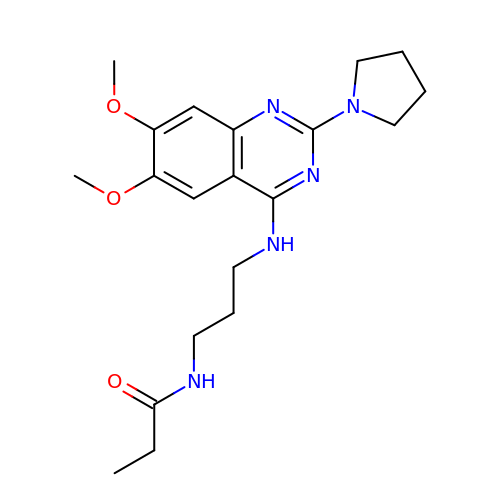N-(3-{[6,7-dimethoxy-2-(pyrrolidin-1-yl)quinazolin-4-yl]amino}propyl)propanamide | C20 H29 N5 O3 | GDDIMJLTIBWEHU-UHFFFAOYSA-N> MTESVGGNKLVDFLVNVQSILNAASVKCHVVDESFPAKFFEKNPDKIYESYCKFIKNRSNSEGLIRNEDKLVLTTINKRFENGE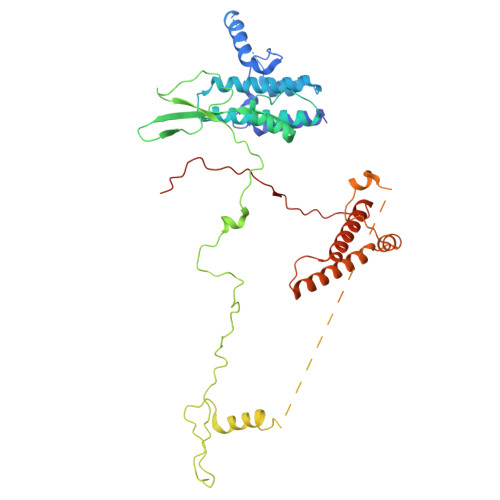YEPIQGGFYKLYHDIKLVCTILIHFYPQGTRNYQLVDKFYKFSSELLLRECCRIGIALTQTNNIKSRSGKLLSGNEMDEYDDDDATELDKIISYDFIKISMNYTVPISQTYQIRTKDMDLFSSIISKSNLDKRPHELPNTNFKINNVLPQTDIENEAPRLGFVGANTSNIPDPTLPPTEMMTRFLHPNWYALPTTVWLKYGNYNSWAPSFNENGTVVDSTTRGLIWLERIGYMDLYEKNEKKVKQEELLNTNEEGINRKQNDENNKNVDGKSNGVQDDGGDNDNDATIASANSESTENKEQFIIKLQNLYNWTPSNYIGDDEIENFRNGTPDKLVSDSLLKLKRLRKERILNKVLKPTTEERELYFKVKRILKEVILAKKVSKVPINNVRAFPVLQTNYNGSIPVVRAQPGRKRKHKK> GGNDFVSRLKALDGREGKIVSSYDDENTGRCRL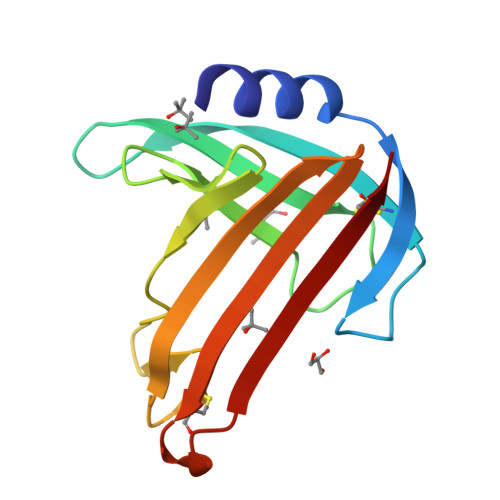ELQKYELEDGSQGLAVYLQDTGMYFTPSAGLDKETKLKDANTAVVSTSSERPGGDACGDFGGALGYKKVLVLKDNQVTIRETFRCVMDGFKKYDLSTTCQF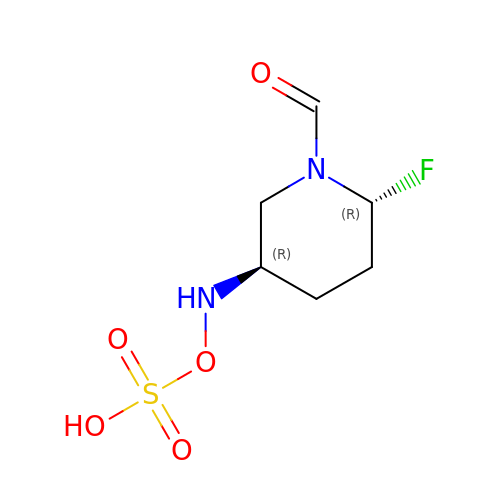[[(3~{R},6~{R})-6-fluoranyl-1-methanoyl-piperidin-3-yl]amino] hydrogen sulfate | C6 H11 F N2 O5 S | NHFNUMMVPZGHRV-RITPCOANSA-N> MGTSRRDWQLQQLGITQWSLRRPGALQGEIAIAIPAHVRLVMVANDLPALTDPLVS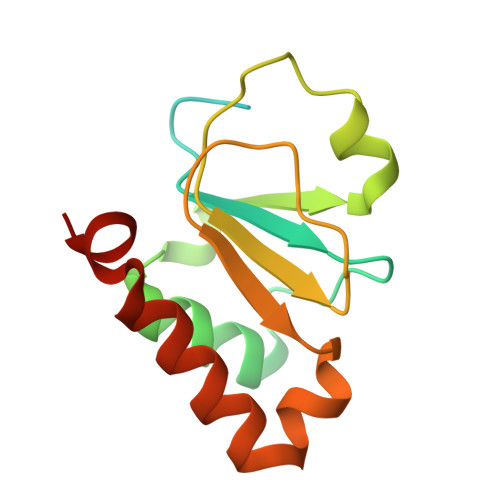DVLRALTVSPDQVLQLTPEKIAMLPQGSHCNSWRLGTDEPLSLEGAQVASPALTDLRANPTARAALWQQICTYEHDFFPRND> MGSSHHHHHHSSGLEVLFQGPHMETAIWIKNSKLPAVLVAAGAFDAAVQALSKQVGVVKLEPLKKYFTNIYEGCRTYIPSTPCELP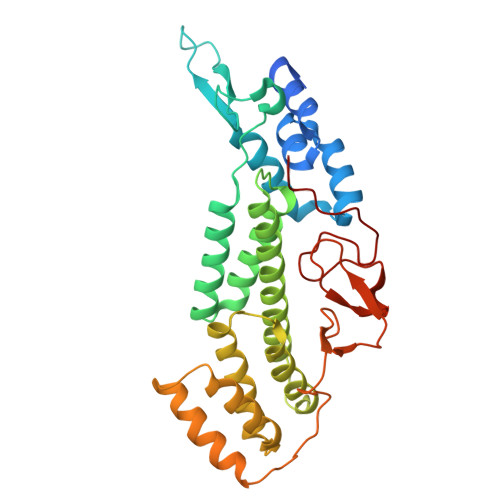AQLGYVRAYDDTVSEDQILPYVPGLDVVNEKMNEGYKNFKLNKPDIAIECFREAIYRITLLMVDDAEDEKLAHKILETAREYILGLSIELERRSLKEGNTVRMLELAAYFTKAKLSPIHRTNALQVAMSQHFKHKNFLQASYFAGEFLKIISSGPRAEQARKIKNKADSMASDAIPIDFDPYAKFDICAATYKPIYEDTPSVSDPLTGSKYVITEKDKIDRIAMISKIGAPASGLRIRV>MKYVVVSGGVISGIGKGVLASSTGMLLKTLGLKVTSIKIDPYMNIDAGTMSPLEHGECFVLDDGGETDLDLGNYERYLGITLSRDHNITTGKIYSHVISRERRGDYLGKTVQIVPHLTNAIQDWIQRVSKIPVDDTGLEPDVCIIELGGTVGDIESAPFVEALRQFQFEVGRENFALIHVSLVPVIHGEQKTKPTQAAIKDLRSLGLIPDMIACRCSEELNRSTIDKIAMFCHVGPEQVVNVHDVNSTYHVPLLLLKQHMIDYLHSRLKLGEVPLTLEDKERGSQLLTNWENMTKNLDDSDDVVKIALVGKY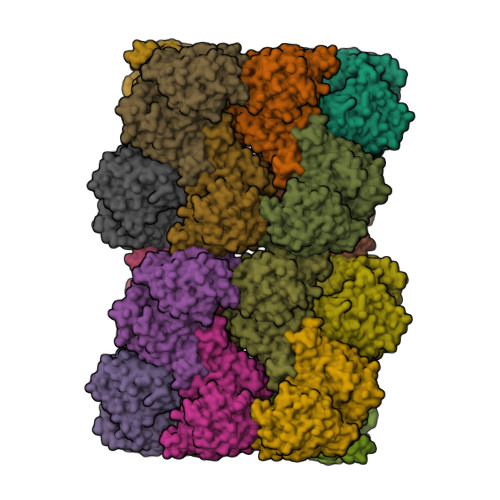TNLKDSYLSVTKSLEHASMKCRRQLEILWVEASNLEPETQEVDKNKFHDSWNKLSSADGILVPGGFGTRGIEGMILAAKWARESGVPFLGVCLGLQVAAIEFARNVIGRPNSSSTEFLDETLLAPEDQVVITMRLGLRPTIFQPNSEWSNIRKLYGEVNEVHERHRHRYEINPKIVNDMESRGFIFVGKDETGQRCEIFELKGHPYYVGTQYHPEYTSKVLEPSRPFWGLVAAASGTLGEVIKDINL[16x]> GAMEPTMDLSAFKDGLEVIVPNPITTLVPSTGYPRPTATWCFGDKVLETGDRVKMKTLSAYAELVISPSERSDKGIYTLKLENRVKTISGEIDVNVIARPSAPKELKFGDITKDSVHLTWEPPDDDGGSPLTGYVVEKREVSRKTWTKVMDFVTDLEFTVPDLVQGKEYLFRVCARNKCGPGEPAYVDEPVNMSTPATVPDPPENVKWRDRTANSIFLTWDPPKNDGGSRIKGYIVERCPRGSDKWVACGEPVAETKMEVTGLEEGKWYAYRVKALNRQGASKPSRPTEEIQAVDTQEAP

Titin is a giant, elastic, sarcomeric protein with a molecular weight of more than 3800 kD. Titin consists primarily of two types of protein domains: fibronectin type III (FnIII) domains and immunoglobulin (Ig) domains (ca 100 residues in length) that account for over 90% of its mass. Despite the repetitive composition of titin, a single main immunogenic region (MIR) has so far been identified in its chain that elicits the reactivity of almost all known anti-titin antibodies in MG patients. This 30 kD segment, also termed MGT30, consists of a domain triplet of composition Ig-FnIII-FnIII located in the titin segment at the junction of the I- and A-bands (I/A) and corresponding to domains 4 to 6 in this region of the chain, i.e., tandem I109-I111 also termed I/A4-I/A6, (nomenclature as in Bang et al., 2001).

To gain an insight into the possible molecular determinants of I110 recognition by anti-titin antibodies, we elucidated the 3D-structure of the isolated I110 domain, the double tandem I110-I111 and the full-length MIR region I109-I110 using X-ray crystallography. The structures showed that the domains contain structure and sequence features typical of Ig and FnIII constituents of titin, and that share high levels of sequence and structural conservation with other domains of titin. I110 is joined to the preceding Ig through a short two-residue linker sequence, residues AM, with the relative orientation of both domains being fixed by two interdomain salt bridges. C-terminally, I110 is joined to the subsequent domain by a flexible three residue long, hydrophilic linker, STA. No direct contacts exist between I110 and I111, so that the linker sequence acts as an effective hinge permitting the free repositioning of both domains. Accordingly, the structures of I110-I111 and I109-I111 show a different mutual arrangement of these domains. Since the crystal structures of MIR domain tandems and isolated I110 show that the structure of I110 is not affected by flanking domains, the apparent reduced binding could be simply due to the specific methodology used. The 3D structure of the titin MIR will help future studies on the pathomechamisms acting in titin-based autoimmunity and should also improve diagnostics for titin antibodies as an important biomarker for thymoma and MG severity diagnosis.>MRSFPKAKEAFSEGEKVSFGVHRLHVGDAREVLASFPEASVHLVVTSPPYWTLKRYEDTPGQLGHIEDYEAFLDELDRVWREVFRLLVPGGRLVIVVGDVAVARRRFGRHLVFPLHADIQVRCRKLGFDNLNPIIWHKHTNASLEVEGRGVFLGKPYEPGAIIKTEIEYILMQRKPGGYRKPTQEQREKSRLPKEDF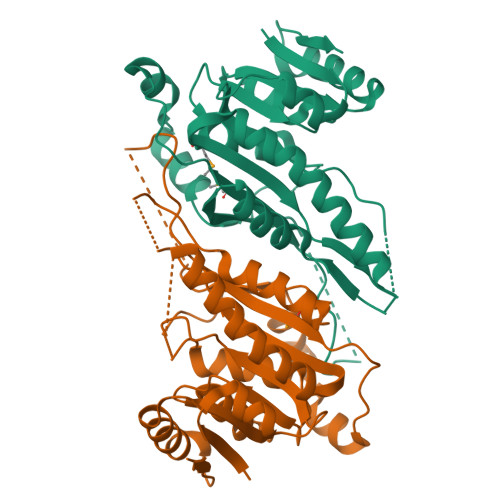HRFFRQIWDDIPGESTKDHPAPFPLELAERLVRMFSFVGDVVLDPFAGTGTTLIAAARWGRRALGVELVPRYAQLAKERFAREVPGFSLEVLDGATHPRR[2x]>[7x]NNNFFDPKLMSDWEDEDLDTDNDNIPDSYERNGYTIKDLIAVKWEDSFAEQGYKKYVSNYLESNTAGDPYTDYEKASGSFDKAIKTEARDPLVAAYPIVG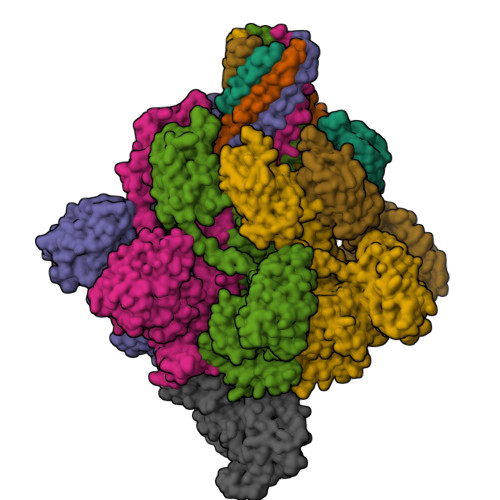VGMEKLIISTNEHASTDQGKTVSRATTNSKTESNTAGVSVNVGYQNGFTANVTTNYSHTTDNSTAVQDSNGESWNTGLSINKGESAYINANVRYYNTGTAPMYKVTPTTNLVLDGDTLSTIKAQENQIGNNLSPGDTYPKKGLSPLALNTMDQFSSRLIPINYDQLKKLDAGKQIKLETTQVSGNFGTKNSSGQIVTEGNSWSDYISQIDSISASIILDTENESYERRVTAKNLQDPEDKTPELTIGEAIEKAFGATKKDGLLYFNDIPIDESCVELIFDDNTANKIKDSLKTLSDKKIYNVKLERGMNILIKTPTYFTNFDDYNNYPSTWSNVNTTNQDGLQGSANKLNGETKIKIPMSELKPYKRYVFSGYSKDPLTSNSIIVKIKAKEEKTDYLVPEQGYTKFSYEFETTEKDSSNIEITLIGSGTTYLDNLSITELNSTPEILDEPEVKIPTDQEIMDAHKIYFADLNFNPSTGNTYINGMYFAPTQTNKEALDYIQKYRVEATLQYSGFKDIGTKDKEMRNYLGDPNQPKTNYVNLRSYFTGGENIMTYKKLRIYAITPDDRELLVLSVD;> APIERPEDFLKDKEKAKEWERKEAERIEQKLERSEKEALESYKKDSVEISKYSQTRNYFYDYQIEANSREKEYKELRNAISKNKIDKPMYVYYFESPEKFAFNKVIRTENQNEISLEKFNEFKETIQNKLFKQDGFKDISLYEPGKGDEKPTPLLMHLKLPRNTGMLPYTNTNNVSTLIEQGYSIKIDKIVRIVIDGKHYIKAEASVVSSLDFKDDVSKGDSWGKANYNDWSNKLTPNELADVNDYMRGGYTAINNYLISNGPVNNPNPELDSKITNIENALKREPIPTNLTVYRRSGPQEFGLTLTSPEYDFNKLENIDAFKSKWEGQALSYPNFISTSIGSVNMSAFAKRKIVLRITIPKGSPGAYLSAIPGYAGEYEVLLNHGSKFKINKIDSYKDGTITKLIVDATLIPENLYFQGLEHHHHHH>MSPSKESDELIFFVNGKKVTERNADPEVNLLFYLRKVIRLTGTKYGCGGGDCGACTVMISRYDPISKRISHFSATACLVPICSLHGAAVTTVEGIGSTKTRIHPVQERIAKGHGTQCGFCTPGMVMSIYTLLRNHPEPSTEQIMETLGGNLCRCTGYRPIVESAKSFCPSSTCCQMNGEGKCCLDEEKNEPERKNSVCTKLYEKKEFQPLDPTQELIFPPELMRMAEESQNTVLTFRGERTTWIAPGTLNDLLELKMKHPSAPLVIGNTYLGLHMKFTDVSYPIIISPARILELFVVTNTKQGLTLGTGLSLTQVKNVLSDVVSRLPKEKTQIYCALLKQLKTLAGQQIRNVASLGGHIISRLPTSDLNPILGIGNCILNVASTEGIQQIPLNDHFLAGVPDAILKPEQVLISVFVPRSSKWEFVSAFRQAPRQQNAFATVNAGMKVVFKEDTNTITDLGILYGGIGATVISADKSCRQLIGRCWDEEMLDDAGKMICEEVSLLMAAPGGMEEYRKTLAISFLFMFYLDVLKQLKTRDPHKYPDISQKLLHILEDFPLTMPYGMQSFQDVDFQQPLQDPIGRPIMHQSGIKHATGEAVFCDDMSVLPGELFLAVVTSSKSHAKIISLDASEALASLGVVDVVTARDV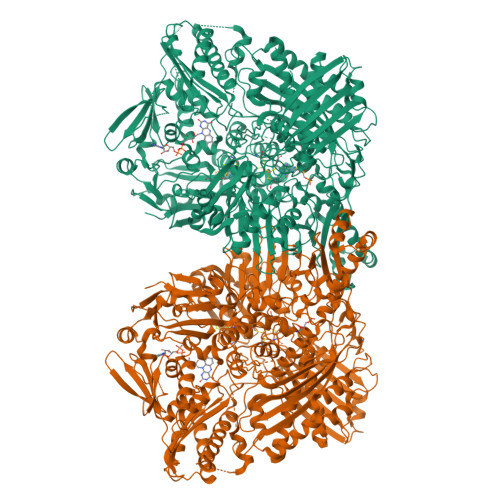PGDNGREEESLYAQDEVICVGQIVCAVAADSYAHAQQAAKKVKIVYQDIEPMIVTVQDALQYESFIGPERKLEQGNVEEAFQCADQILEGEVHLGGQEHFYMETQSVRVVPKGEDKEMDIYVSSQDAAFTQEMVARTLGIPKNRINCHVKRVGGAFGGKASKPGLLASVAAVAAQKTGRPIRFILERRDDMLITGGRHPLLGKYKIGFMNNGKIKAADIQLYINGGCTPDDSELVIEYALLKLENAYKIPNLRVRGRVCKTNLPSNTAFRGFGFPQGAFVTETCMSAVAAKCRLPPEKVRELNMYRTIDRTIHNQEFDPTNLLQCWEACVENSSYYNRKKAVDEFNQQRFWKKRGIAIIPMKFSVGFPKTFYYQAAALVQIYTDGSVLVAHGGVELGQGINTKMIQVASRELKIPMSYIHLDEMSTVTVPNTVTTGASTGADVNGRAVQNACQILMKRLEPIIKQNPSGTWEEWVKEAFVQSISLSATGYFRGYQADMDWEKGEGDIFPYFVFGAACSEVEIDCLTGAHKNIRTDIVMDGSFSINPAVDIGQIEGAFVQGLGLYTLEELKYSPEGVLYTRGPHQYKIASVTDIPEEFHVSLLTPTPNPKAIYSSKGLGEAGTFLGCSVFFAIAAAVAAAREERGLSPIWAINSPATAEVIRMACEDQFTNLVPQTDSKCCKPWSIPVA[4x]> MDSQGLKTAVAIFLATTFSATSYQACSAGPDTAPSLTVQQSNALPTWWKQAVFYQVYPRSFKDTNGDGIGDLNGIIENLDYLKKLGIDAIWINPHYDSPNTDNGYDIRDYRKIMKEYGTMEDFDRLISEMKKRNMRLMIDIVINHTSDQHAWFVQSKSGKNNPYRDYYFWRDGKDGHAPNNYPSFFGGSAWEKDDKSGQYYLHYFAKQQPDLNWDNPKVRQDLYDMLRFWLDKGVSGLRFDTVATYSKIPNFPDLSQQQLKNFAEEYTKGPKIHDYVNEMNREVLSHYDIATAGEIFGVPLDKSIKFFDRRRNELNIAFTFDLIRLDRDADERWRRKDWTLSQFRKIVDKVDQTAGEYGWNAFFLDNHDNPRAVSHFGDDRPQWREHAAKALATLTLTQRATPFIYQGSELGMTNYPFKKIDDFDDVEVKGFWQDYVETGKVKAEEFLQNVRQTSRDNSRTPFQWDASKNAGFTSGTPWLKINPNYKEINSADQINNPNSVFNYYRKLINIRHDIPALTYGSYIDLDPDNNSVYAYTRTLGAEKYLVVINFKEEVMHYTLPGDLSINKVITENNSHTIVNKNDRQLRLEPWQSGIYKLNP

SIases, classified as glycoside hydrolase family 13 (GH13) enzymes, catalyze the isomerization of sucrose to produce isomaltulose and trehalulose as primary products and D-glucose and D-fructose as by-products. NX-5 (named NX-5 in this work) that predominantly produces isomaltulose (~87%). Similar to other GH13 family enzymes, the NX-5 molecule is composed of three domains: the N-domain (residues 42-145 and 216-520), the sub-domain (residues 146-215), and the C-domain (residues 521-600). Among them, residues Asp102, His145, Arg239, His368, Asp369, Glu428, and Arg456 are responsible for sucrose binding and residues Asp241 (the nucleophile) and Glu295 (the acid catalyst) are crucial for sucrose hydrolysis for PalI, MutB, and SmuA.

Crystals of NX-5 diffracted to 1.70 Å resolution and belonged to the space group P2 12 121, with unit-cell parameters a = 58.9 Å, b = 81.3 Å, c = 138.0 Å. There is one molecule in the asymmetric unit of the crystal lattice. The final model included residues 42-600 of NX-5 and two glycerol molecules while the electron density for the C-terminal His-tag was not visible. A hexa-coordinate magnesium ion was found to interact with five residues (Asp63, Asn65, Asp67, Ile69, and Asp71) highly conserved in all known SIases. In the NX-5 structure, the magnesium ion was about 23 Å away from the active site pocket, suggesting its function may be structural rather than catalytic. The active site of NX-5 is located in a pocket that is approximately 25 Å deep from the negatively charged surface. Similar to the function of the corresponding residues Phe256/Phe270 and Phe280/Phe294 in MutB/SmuA, Phe297 and Phe321 in NX-5 form an aromatic clamp near the entrance of the active pocket. Phe321 and Phe297 in NX-5 are closer to the catalytic325RLDRD329 motif and residue Glu295. Superimposition of 15 residues (Asp102, His145, Gln209, Arg239, Ala241, Glu295, Phe297, Phe321, Arg325, Arg328, Arg333, His368, Asp369, Glu428 and Arg456) in the substrate-binding pocket of the native NX-5, the E295Q/sucrose complex and the D241A/glucose complex show subtle structural changes in the active site pocket with an RMSD of 0.20 Å between the native NX-5 and the E295Q/sucrose complex and an RMSD of 0.15 Å between the native NX-5 and the D241A/glucose complex.N~6~-methyl-N~6~-[4-(trifluoromethoxy)phenyl]pyrido[3,2-d]pyrimidine-2,4,6-triamine 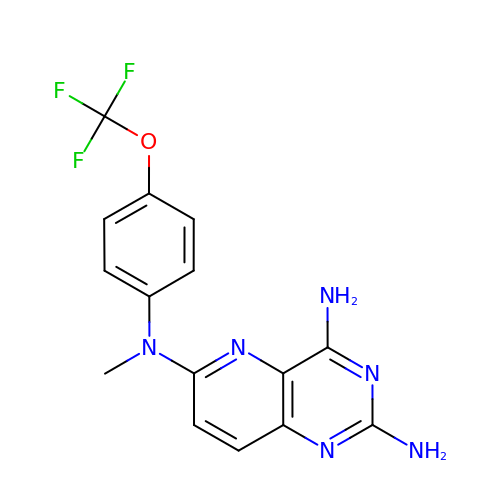| C15 H13 F3 N6 O | JEGBSKQTMYWCPV-UHFFFAOYSA-N3,5,7-TRIHYDROXY-2-(3,4,5-TRIHYDROXYPHENYL)-4H-CHROMEN-4-ONE | C15 H10 O8 | 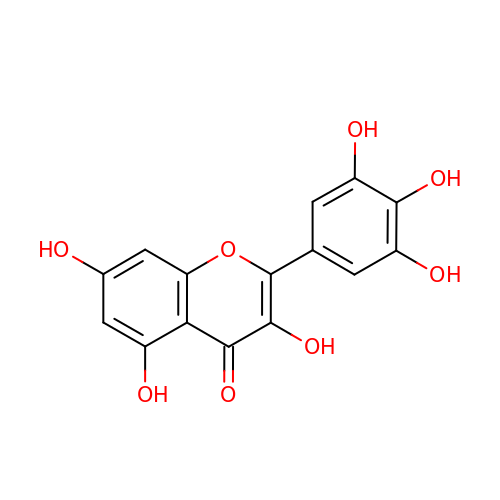IKMDFBPHZNJCSN-UHFFFAOYSA-N> MDDGRKKELHDLNTRAWNGEEVFPLKSKKLDSSIKRNTGFIKKLKKGFVKGSESSLLKDLSEASLEKYLSEIIVTVTECLLNVLNKNDDVIAAVEIISGLHQRFNGRFTSPLLGAFLQAFENPSVDIESE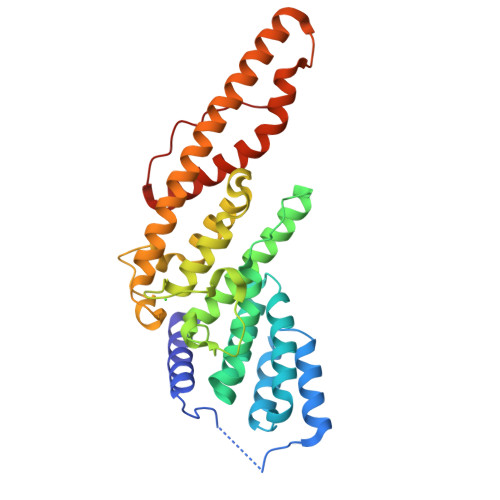RDELQRITRVKGNLRVFTELYLVGVFRTLDDIESKDAIPNFLQKKTGRKDPLLFSILREILNYKFKLGFTTTIATAFIKKFAPLFRDDDNSWDDLIYDSKLKGALQSLFKNFIDATFARATELHKKVNKLQREHQKCQIRTGKLRDEYVEEYDKLLPIFIRFKTSAITLGEFFKLEIPELHHHHHH>[2x]SKLQATKTLAADVIMRSPVSWKQELTLDAGRSKGASENMLAIANGGLIGSVSKVEENSTIVNLLTNTENADKISVKIQHG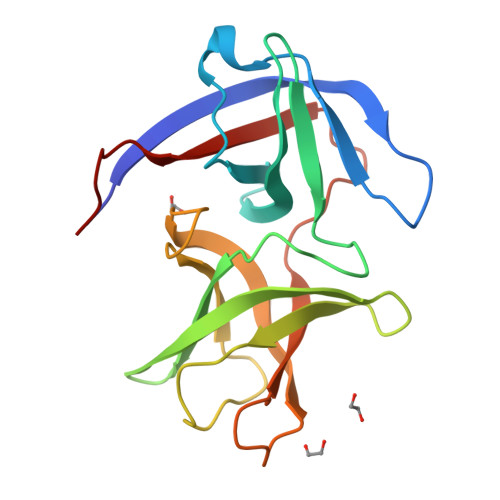STTIYGIIIGYDKENDVLKISQLNSNSDISAGDKVTTGGLGNFNVADIPVGEVVATTHSTDYLTREVTVKLSADTHNVDVIELVGNSKLVPR>GAMETITVPTPIKQIFSDDAFAETIKDNLKKKSVTDAVTQNELNSIDQIIANNSDIKSVQGIQYLPNVTKLFLNGNKLTDIKPLANLKNLGWLFLDENKVKDLSSLKDLKKLKSLSLEHNGISDINGLVHLPQLESLYLGNNKITDITVLSRLTKLDTLSLEDNQISDIVPLAGLTKLQNLYLSKNHISDLRALAGLKNLDVLELFSQECLNKPINHQSNLVVPNTVKNTDGSLVTPEIISDDGDYEKPNVKWHLPEFTNEVSFIFYQPVTIGKAKARFHGRVTQPLKE[2x];>ETRECKEALAKSEMNVNMKCQLPNFTAETPIQNVILHEHHIFLGATNYIYVLNEEDLQKVAEYKTGPVLEHPDCFPCQDCSSKANLSGGVWKDNINMALVVDTYYDDQLISCGSVNRGTCQRHVFPHNHTADIQSEVHCIFSPQIEEPSQCPDCVVSALGAKVLSSVKDRFINFFVGNTINSSYFPDHPLHSISVRRLKETKDGFMFLTDQSYIDVLPEFRDSYPIKYVHAFESNNFIYFLTVQRETLDAQTFHTRIIRFCSINSGLHSYMEMPLECILTEKRKKRSTKKEVFNILQAAYVSKPGAQLARQIGASLNDDILFAVFAQSKPDSAEPMDRSAMCAFPIKYVNDFFNKIVNKNNVRCLQHFYGPNHEHCFNRTLLRNSSGCEARRDEYRTEFTTALQRVDLFMGQFSEVLLTSISTFIKGDLTIANLGTSEGRFMQVVVSRSGPSTPHVNFLLDSHPVSPEVIVEHTLNQNGYTLVITGKKITKIPLNGLGCRHFQSCSQCLSAPPFVQCGWCHDKCVRSEECLSGTWTQQICLPAIYKVFPNSAPLEGGTRLTICGWDFGFRRNNKFDLKKTRVLLGNESCTLTLSESTMNTLKCTVGPAMNKHFNMSIIISNGHGTTQYSTFSYVDPVITSI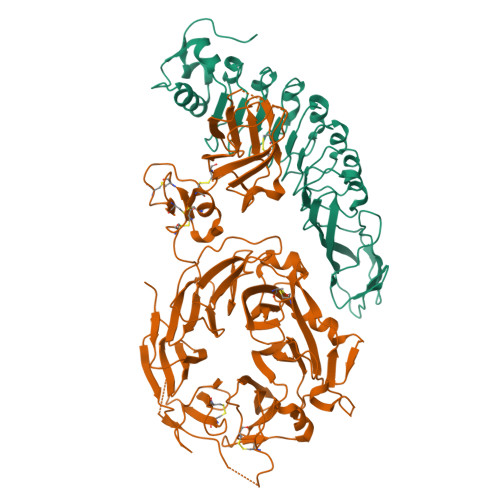SPKYGPMAGGTLLTLTGNYLNSGNSRHISIGGKTCTLKSVSNSILECYTPAQTISTEFAVKLKIDLANRETSIFSYREDLHHHHHH[2x]> NALLRYLLD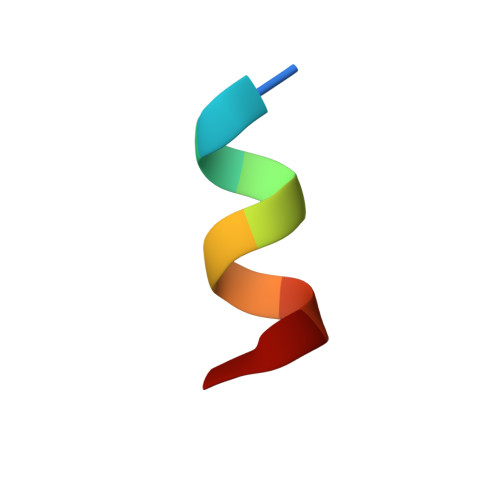K>[2x]ENLYFQGHMIKSIPEWSEQEYLMLSLPHEKSDWNPYLEEILQSYKEFVKVVSEFQKVLLIAPKQSDFENFK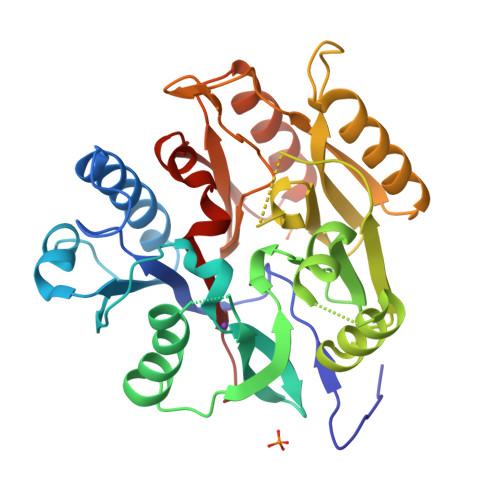DIKNVEFFKCDTNDTWIRDFGAIDIVENGRLKALDFTFNAWGNKFQSELDNAVNSKLFKEKFKEELKKVDFILEGGSIDFNGEGVMLTSSHCLLNENRNSHLNKTQIDTKLKEIFGLKQIIWLENGFIKGDDTDHHIDTLARFIDKNTIAHCICEDEEDEHYLPLQKMKEELKKTGFDLLELPIPKPLYYEERRLGATYANFVFINNALIVPFYKDKNDEIIAKRLSKALPNHKIIGVDARVFLRQNGSLHCSCQNRFKGLR> REFTIDFSTQQSYVSSLNSIRTEISTPLEHISQGTTSVSVINHTPPGSYFAVDIRGLDVYQARFDHLRLIIEQNNLYVAGFVNTATNTFYRFSDFTHISVPGVTTVSMTTDSSYTTLQRVAALERSGMQISRHSLVSSY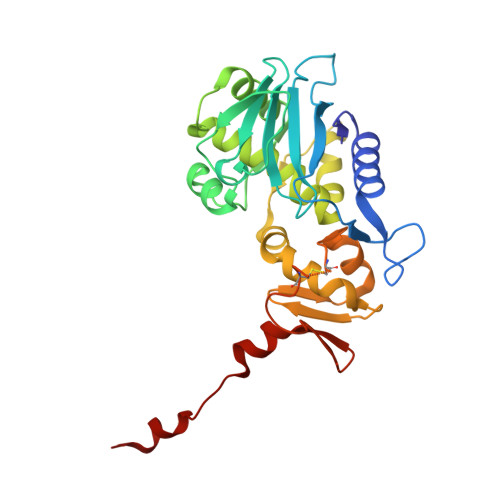LALMEFSGNTMTRDASRAVLRFVTVTAEALRFRQIQREFRQALSETAPVYTMTPGDVDLTLNWGRISNVLPEYRGEDGVRVGRISFNNISAILGTVAVILNCHHQGARSVRAVNEDSQPECQITGDRPVIKINNTLWESNTAAAFLNRKSQFLYTTGK> QGPDSMKKDVPPSINTTNIDTLLVATDQTERIVEPPENIQEKIAFIFNNLSQSNMTQKVEELKETVKEEFMPWVSQYLVMKRVSIEPNFHSLYSNFLDTLKNPEFNKMVLNETYRNIKVLLTSDKAAANFSDRSLLKNLGHWLGMITLAKNKPILHTDLDVKSLLLEAYVKGQQELLYVVPFVAKVLESSIRSVVFRPPNPWTMAIMNVL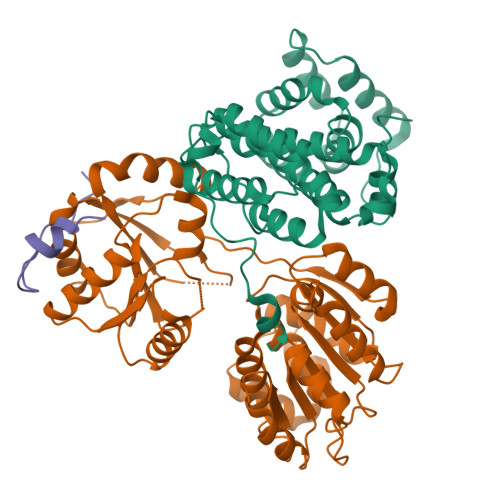AELHQEHDLKLNLKFEIEVLCKNLALDINELKPGNLLKDKDRLKNLDE;> RSMGNEFEDYCLKRELLMGIFEMGWEKPSPIQEESIPIALSGRDILARAKNGTGKSGAYLIPLLERLDLKKDNIQAMVIVPTRELALQVSQICIQVSKHMGGAKVMATTGGTNLRDDIMRLDDTVHVVIATPGRILDLIKKGVAKVDHVQMIVLDEADKLLSQDFVQIMEDIILTLPKNRQILLYSATFPLSVQKFMNSHLQKPYEINLMEELTLKGVTQYYAYVTERQKVHCLNTLFSRLQINQSIIFCNSSQRVELLAKKISQLGYSCFYIHAKMRQEHRNRVFHDFRNGLCRNLVCTDLFTRGIDIQAVNVVINFDFPKLAETYLHRIGRSGRFGHLGLAINLITYDDRFNLKSIEEQLGTEIKPIPSNIDKSLY;> RSMGDSKRVFGERRRNDSYTEEEPEWFSAGPTSQSETIELTGFD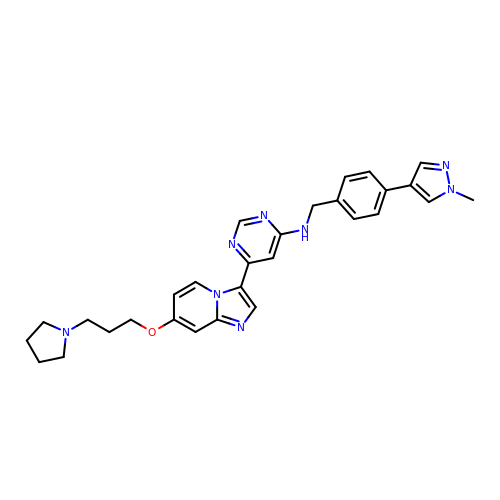~{N}-[[4-(1-methylpyrazol-4-yl)phenyl]methyl]-6-[7-(3-pyrrolidin-1-ylpropoxy)imidazo[1,2-a]pyridin-3-yl]pyrimidin-4-amine | C29 H32 N8 O | LVMAULGVWBINFP-UHFFFAOYSA-N(4bS,6S)-6-methoxy-1,4,6,7,9,10,12,13-octahydro-3H,5H-pyrano[4',3':3,4]pyrido[2,1-i]indol-3-one | C16 H21 N O3 | 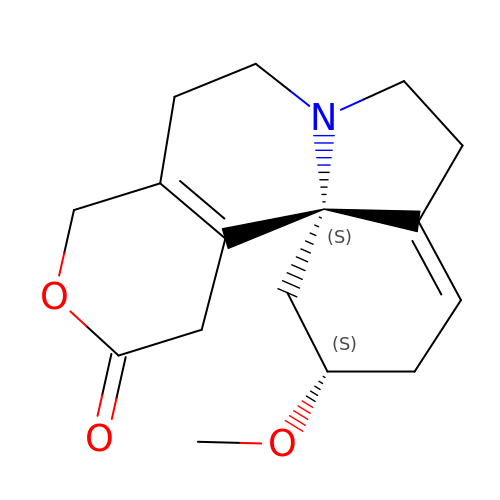ALSKYCOJJPXPFS-BBRMVZONSA-N> NNVENEKSWEKYFAEYKVEGCFMLFNNSQGTFKVYNLERSQQRFLPASTFKIFNSLVGLETGVIKDTSFVIPWDGVTRDMPEWNHDLSMQQAFRVSAVPYFQEVARRITKPVMQHWLDTVKFGNMKISKIDTFWLDNSLQISPDEELGFVKKLYFDQLPFHKVTMQNVRQVMLMEKKPEYELSYKTGMGFSGPKTIGWITGWIEENGHPSFFVLNIE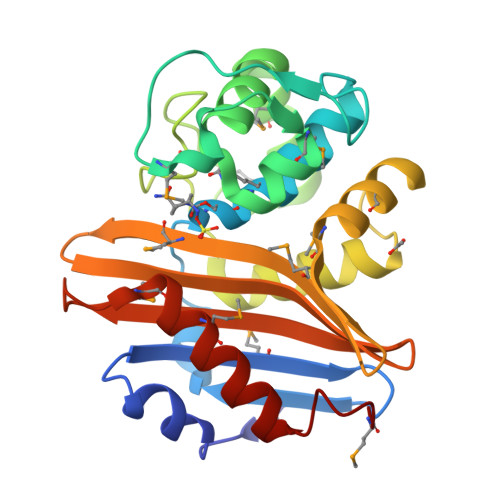TENKSLDMRTVRMNILRNLLTDAGYFKGMK>PTYPKYLLSPETIEALRKPTFDVWLWEPNEMLSCLEHMYHDLGLVRDFSINPVTLRRWLFCVHDNYRNNPFHNFRHCFCVAQMMYSMVWLCSLQEKFSQTDILILMTAAICHDLDHPGYNNTYQINARTELAVRYNDISPLENHHCAVAFQILAEPECNIFSNIPPDGFKQIRQGMITLILATDMARHAEIMDS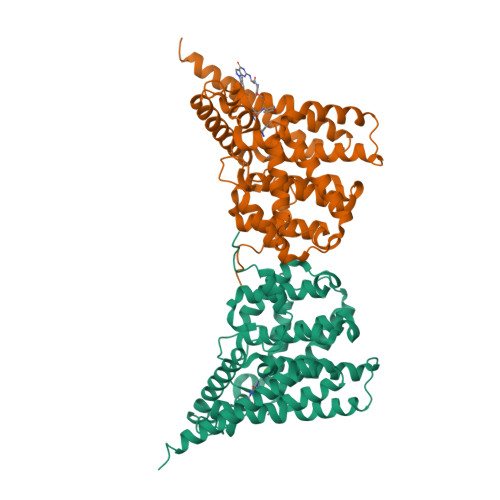FKEKMENFDYSNEEHMTLLKMILIKCCDISNEVRPMEVAEPWVDCLLEEYFMQSDREKSEGLPVAPFMDRDKVTKATAQIGFIKFVLIPMFETVTKLFPMVEEIMLQPLWESRDRYEELKRIDDAMKELQKK[2x]> GSMENTDVFLGLHDFLERMRKPSAGDFVKSIKSFIVSFSNNAPDPEKDCAMVQEFFSKME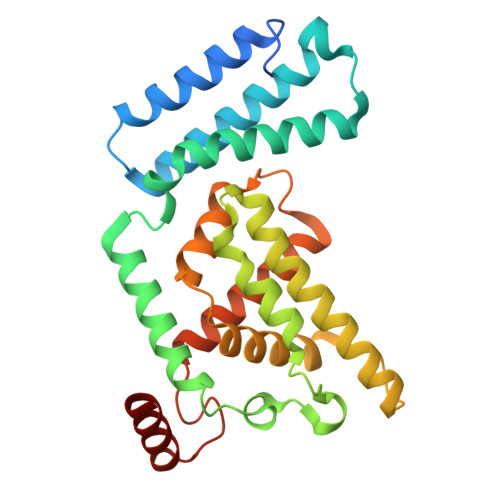AAFRAHPLWSGCSEEELDSAGDGLEKYVMTKLFTRVFASNTEEVIADEKLFQKMSLVQQFISPENLDIQPTFQNESSWLLAQKELQKINMYKAPRDKLVCILNCCKVINNLLLNASIASNENAPGANEFLPVLIYVTIKANPPQLHSNLLYIQRYRRESKLVGEAAYFFTNILSAESFISNIDAKSISLDEAEFEKNMESARARISG> MASTPRIVIIGAGIVGTNLADELVTRGWNNITVLDQGPLNMPGGSTSHAPGLVFQTNPSKTMASFAKYTVEKLLSLTEDGVSCFNQVGGLEVATTETRLADLKRKLGYAAAWGIEGRLLSPAECQELYPLLDGENILGGLHVPSDGLASAARAVQLLIKRTESAGVTYRGSTTVTGIEQSGGRVTGVQTADGVIPADIVVSCAGFWGAKIGAMIGMAVPLLPLAHQYVKTTPVPAQQGRNDQPNGARLPILRHQDQDLYYREHGDRYGIGSYAHRPMPVDVDTLGAYAPETVSEHHMPSRLDFTLEDFLPAWEATKQLLPALADSEIEDGFNGIFSFTPDGGPLLGESKELDGFYVAEAVWVTHSAGVAKAMAELLTTGRSETDLGECDITRFEDVQLTPEYVSETSQQNFVEIYDVLHPLQPRLSPRNLRVSPFHARHKELGAFFLEAGGWERPYWFEANAALLKEMPAEWLPPAR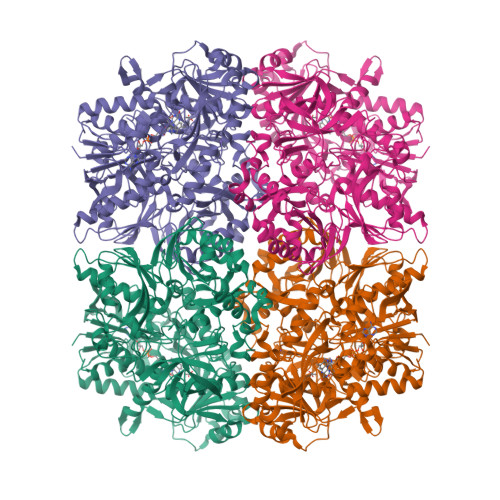DAWSGMFSSPIAAAEAWKTRTAVAMYDMTPLKRLEVSGPGALKLLQELTTADLAKKPGAVTYTLLLDHAGGVRSDITVARLSEDTFQLGANGNIDTAYFERAARHQTQSGSATDWVQVRDTTGGTCCIGLWGPLARDLVSKVSDDDFTNDGLKYFRAKNVVIGGIPVTAMRLSYVGELGWELYTSADNGQRLWDALWQAGQPFGVIAAGRAAFSSLRLEKGYRSWGTDMTTEHDPFEAGLGFAVKMAKESFIGKGALEGRTEEASARRLRCLTIDDGRSIVLGKEPVFYKEQAVGYVTSAAYGYTVAKPIAYSYLPGTVSVGDSVDIEYFGRRITATVTEDPLYDPKMTRLRG>MKTLTEIKQTPKGIIKADESFNQVKDKIRLPRRILYLGCGSSHFLAKLLAMVTNMHGGTGVALPCSEFLYSKEAYPIGKPELVVGISRSGETTEVLLALEKINTPKLGISAYESSLTRACDYSLVVPTIEESVVMTHSFTAFYFAYLQLLRHSYGLPLLEATEVAKATEKALEYENYIKEIVEDFDFQNVIFLGSGLLYPVALEASLKMKEMAIFWSEAYPTFEVRHGFKAIADENTLVVLMAQELFEWHKKLVNEFKGQRARVLLISNSQQEFGQ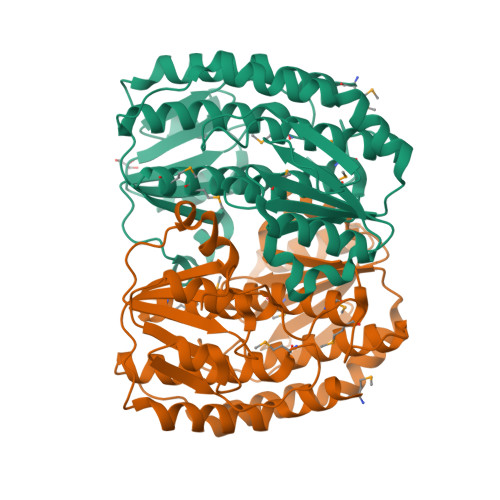DYSIEVPRLSKDATPIPYLPVVQLLSYYKAVARGLNPDNPRFLDKVVRWLEHHHHHH[2x]> SQIRQNYSTEVEAAVNRLVNLYLRASYTYLSLGFYFDRDDVALEGVCHFFRELAEEKREGAERLLKMQNQRGGRALFQDLQKPSQDEWGTTLDAMKAAIVLEKSLNQ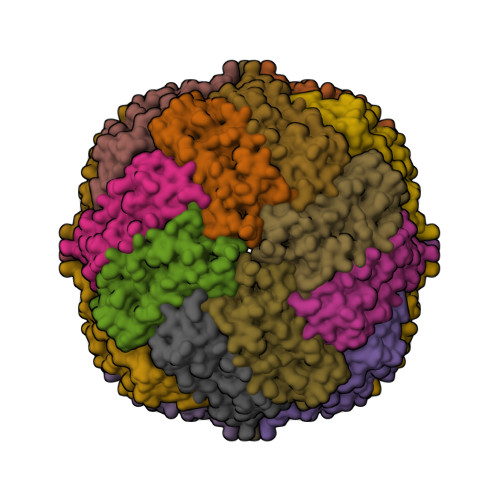ALLDLHALGSAQADPHLCDFLESHFLDEEVKLIKKMGDHLTNIQRLVGSQAGLGEYLFERLTL>[2x]MNSKCHCVILNDGNFIPVLGFGTALPLECPKSKAKELTKIAIDAGFHHFDSASVYNTEDHVGEAIRSKIADGTVRREDIFYTSKVWCTSLHPEL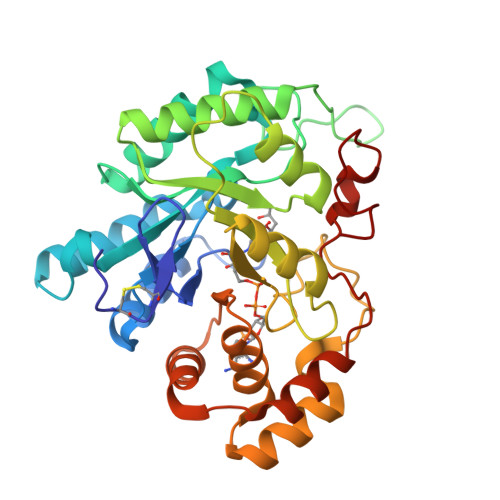VRASLERSLQKLQFDYVDLYLIHYPMALKPGEENFPVDEHGKLIFDRVDLCATWEAMEKCKDAGLTKSIGVSNFNYRQLEMILNKPGLKYKPVCNQVECHPYLNQMKLLDFCKSKDIVLVAYGVLGTQRYGGWVDQNSPVLLDEPVLGSMAKKYNRTPALIALRYQLQRGIVVLNTSLKEERIKENMQVFEFQLSSEDMKVLDGLNRNMRYIPAAIFKGHPNWPFLDEY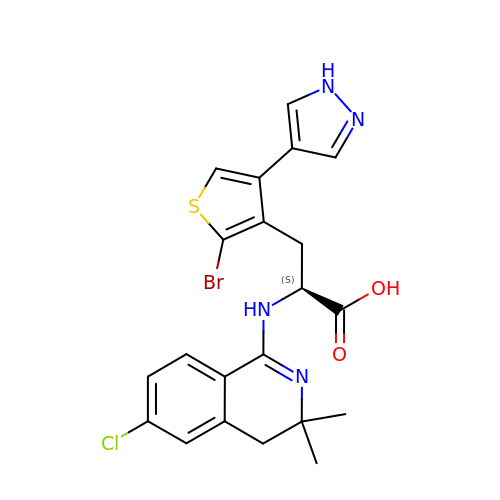3-[2-bromo-4-(1H-pyrazol-4-yl)thiophen-3-yl]-N-(6-chloro-3,3-dimethyl-3,4-dihydroisoquinolin-1-yl)-L-alanine | C21 H20 Br Cl N4 O2 S | DZVYKFXCGGLAAX-KRWDZBQOSA-N> VTYNLEKRPTTIVLINDTPLNVLLDTGADTSVL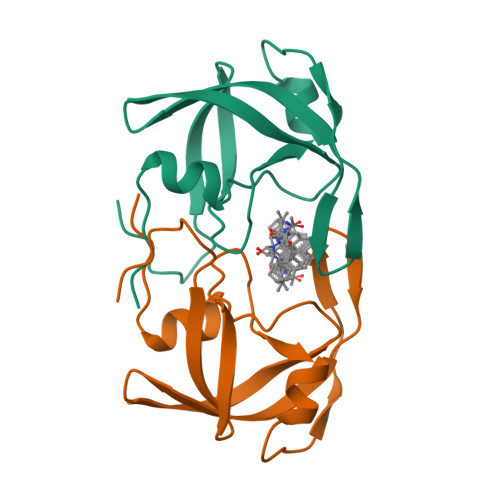TTAHYNRLKYRGRKYQGTGIGGVGGNVETFSTPVTIKKKGRHIKTRMLVADIPVTILGRDILQDLGAKLVL> SLGLQDFDLLRVIGRGSYAKVLLVRLKKTDRIYAMKVVKKELVNDDEDIDWVQTEKHVFEQASNHPFLVGLHSCFQTESRLFFVIEYVNGGDLMFHMQRQRKLPEEHARFYSAEISLALNYLHERGIIYRDLKLDNVLLDSEGHIKLTDYGMCKEGLRPGDTTSTFCGTPNYIAPEILRGEDYGFSVDWWALGVLMFEMMAGRSPFDIVGSSDNPDQNTEDYLFQVILEKQIRIPRSLSVKAASVLKSFLNKDPKERLGCHPQTGFADIQGHPFFRNVDWDMMEQKQVVPPFKPNISGEFGLDNFDSQFTNEPVQLTPDDDDIVRKIDQSEFEGFEYI;> REKLKQELFAFNKTVEHGFPNQPSALAFDPELRIMAIGTRSGAVKIYGAPGVEFTGLHRDAATVTQMHFLTGQGRLLSLLDDSSLHLWEIVHHNGCAHLEEALSFQLPSRPGFDGASAPLSLTRVTVVLLVAAGDIAALGTEGSSVFFLDVTTLTLLEGQTLAPGEVLRSVPDDYRCGKALGPVESLQGHLRDPTKILIGYSRGLLVIWNQASQCVDHIFLGNQQLESLCWGRDSSTVVSSHSDGSYAVWSVDAGSFPTLQPTVATTPYGPFPCKAINKILWRNCESGGHFIIFSGGMPRASYGDRHCVSVLRAETLVTLDFTSRIIDFFTVHSTRPEDEFDDPQALAVLLEEELVVLDLQTPGWPAVPAPYLAPLHSSAITCSAHVASVPAKLWARIVSAGEQQSPQPVSSALSWPITGGRNLAQEPSQRGLLLTGHEDGTVRFWDASGVALRPLYKLSTAGLFQTDCEHADSLAQAAEDDWPPFRKVGCFDPYSDDPRLGVQKVALCKYTAQMVVAGTAGQVLVLELSDVPVEQAVSVAIIDLLQDREGFTWKGHERLSPRTGPLPWPAGFQPRVLVQCLPPAAVTAVTLHTEWSLVAFGTSHGFGLFDYQRKSPVLARCTLHPNDSLAMEGPLSRVKSLKKSLRQSFRRIRKSRVSGKKRAANASSKLQEANAQLAEQACPHDVEMTPVQRRIEPRSADDSLSGVVRCLYFADTFLRDGAHHGPTMWAGTNSGSVFAYALEVPAAAVGGEKRPEQAVEAVLGKEVQLMHRAPVVAIAVLDGRGRPLPEPYEASRDLAQAPDMQGGHAVLIASEEQFKVFTLPKVSAKTKFKLTAHEGCRVRKVALATFASVACEDYAETCLACLTNLGDVHVFSVPGLRPQVHYSCIRKEDISGIASCVFTRHGQGFYLISPSEFERFSLSARNITEPLCSLDI;> THRRVRLHKHGSDRPLGFYIRDGMSVRVAPQGLERVPGIFISRLVRGGLAESTGLLAVSDEILEVNGIEVAGKTLDQVTDMMVANSHNLIVTVKPANQR

The mutually antagonistic relationship of atypical protein kinase C (aPKC) and partitioning-defective protein 6 (Par6) with the substrate lethal giant larvae (Lgl) is essential for regulating polarity across many cell types. Although aPKC–Par6 phosphorylates Lgl at three serine sites to exclude it from the apical domain, aPKC–Par6 and Lgl paradoxically form a stable kinase–substrate complex, with conflicting roles proposed for Par6. Lgl has a double β-propeller structure and contains multiple phosphorylation sites for aPKC–Par6, with at least three serine phospho-acceptor sites (S655, S659 and S663 in human Llgl1, within a segment defined hereafter as the P-site) that map within a key membrane-binding loop13. The structure reveals the intricate interplay between aPKC–Par6 and its substrate Lgl, which, together with in vitro and in vivo data, supports a capture-and-release mechanism involving a stable phospho-intermediate.

The structure of the human aPKCι–Par6α–Llgl1 polarity complex was then determined at a nominal resolution of 3.44 Å using cryo-electron microscopy (cryo-EM). The nucleotide pocket was occupied with adenylyl imidodiphosphate (AMP-PNP) added to the sample before grid preparation to stabilize the kinase core. Two known phospho-threonine sites in aPKC (aPKCιpT412 and aPKCι pT564) and one phospho-serine in Llgl1 (Llgl1pS663) were unequivocally identified from the cryo-EM map. The resulting aPKCι–Par6α–Llgl1 structure reveals the basis for coordinated capture of Llgl1 by Par6α and aPKCι, leading to a stably associated (trapped) phospho-intermediate of Llgl1. The second β-propeller of Llgl1 makes the largest contact with an aPKC-isozyme specific sequence insert (residues G457–D468). A second Llgl1–aPKCιKD contact involves the aPKC RIPR motif (residues R480–R483) in the loop between the αG-helix and αH-helix, also at the base of the kinase C-lobe. The C terminus of the Llgl1 loop (10–11) is bound to the Par6αPDZ domain through a previously unrecognized internal PDZ-binding motif (Llgl1PBM) spanning residues V706–P712. Second, it brings two segments of the loop into close proximity to bridge between aPKCιKD and Par6PDZ by forming a molecular ‘plug’ domain nucleated around the single-site phosphorylation at Llgl1pS663. The phospho-S663 site (Llgl1pS663) identified in the cryo-EM potential map forms a salt bridge with Llgl1R661, which packs against the Llgl1F664 side chain. By forming the plug domain around Llgl1pS663, the P-site effectively blocks access of S655 and S659 phospho-acceptor sites to the aPKCι substrate cleft and catalytic residues.> KKKRLTKADIGTPSNF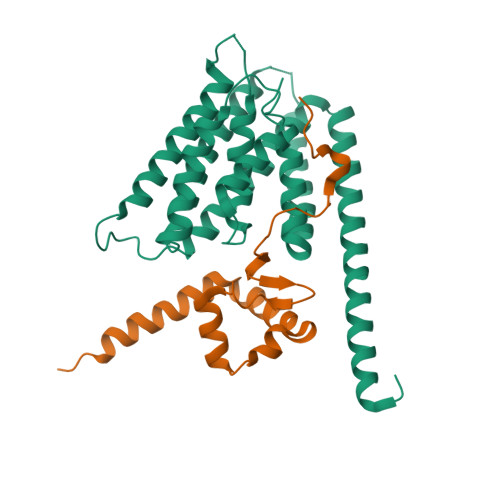QHIGHVGWDPNTGFDLNNLDPELKNLFDMCGISEAQLKDRETSKVIYDFIEKTGGVEAVKNELRRQAENLYFQGLEH;> MGKKSPDSSQGASGPAMQSPSGPTIRPTRPAPPPPTTGGANAKRPATHGKGRAPQPPTAGSSSGSEQPTAMSSEVAKLVSELKDAVHSHAESQKVLKKVSQELQTKWTDWENNRGPDYLLHGYRVIARALQQTYTEQSMLIEGTSSTGPVPQAVTVAKDAVTQTVRGAIKNLENPKPGNDPDGVLMQVVISLGIEGPTLDPGESIQNFLETRVSDFGGDDSDIDYTSDIARLGSALDRVRENHPNEMPRIWIALARELGAAVHSHATSVRIANAGKNHTRDVVRMANESSRLLQGMKVLSVGAWANTMTVLIGDLFEHHHHHHHHH2-azanylethyl-[(2~{S})-2,3-di(hexadecanoyloxy)propoxy]phosphinic acid | C37 H74 N O7 P | 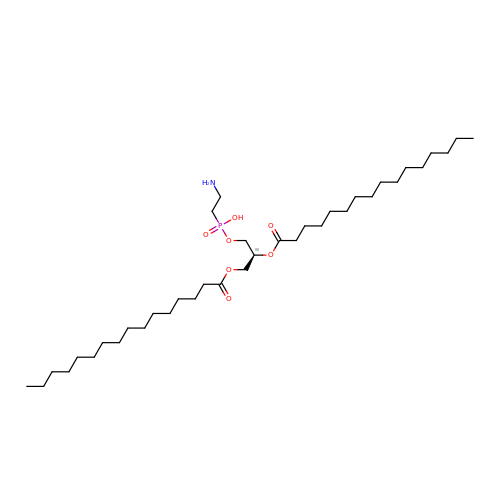BZYHDQIJHNPDON-DHUJRADRSA-N>MAHHHHHHHHHHSGRAEDKSKRDSIEMSMKGCQTNNGFVHNEDILEQTPDPGSSTDNLKHSTRGILGSQEPDFKGVQPYAGMPKEVLFQFSGQARYRIPREILFWLTVASVLVLIAATIAIIALSPKCLDWWQEGPMYQIYPRSFKDSNKDGNGDLKGIQDKLDYITALNIKTVWITSFYKSSLKDFRYGVEDFREVDPIFGTMEDFENLVAAIHDKGLKLIIDFIPNHTSDKHIWFQLSRTRTGKYTDYYIWHDCTHENGKTIPPN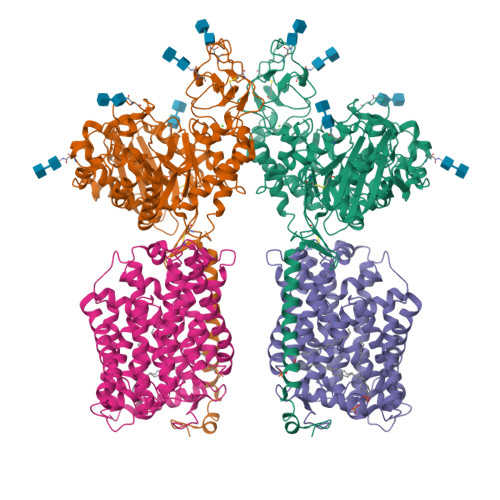NWLSVYGNSSWHFDEVRNQCYFHQFMKEQPDLNFRNPDVQEEIKEILRFWLTKGVDGFSLDAVKFLLEAKHLRDEIQVNKTQIPDTVTQYSELYHDFTTTQVGMHDIVRSFRQTMDQYSTEPGRYRFMGTEAYAESIDRTVMYYGLPFIQEADFPFNNYLSMLDTVSGNSVYEVITSWMENMPEGKWPNWMIGGPDSSRLTSRLGNQYVNVMNMLLFTLPGTPITYYGEEIGMGNIVAANLNESYDINTLRSKSPMQWDNSSNAGFSEASNTWLPTNSDYHTVNVDVQKTQPRSALKLYQDLSLLHANELLLNRGWFCHLRNDSHYVVYTRELDGIDRIFIVVLNFGESTLLNLHNMISGLPAKMRIRLSTNSADKGSKVDTSGIFLDKGEGLIFEHNTKNLLHRQTAFRDRCFVSNRACYSSVLNILYTSC[2x];>MADYKDDDDKSGPDEVDASGRGDTGLRKRREDEKSIQSQEPKTTSLQKELGLISGISIIVGTIIGSGIFVSPKSVLSNTEAVGPCLIIWAACGVLATLGALCFAELGTMITKSGGEYPYLMEAYGPIPAYLFSWASLIVIKPTSFAIICLSFSEYVCAPFYVGCKPPQIVVKCLAAAAILFISTVNSLSVRLGSYVQNIFTAAKLVIVAIIIISGLVLLAQGNTKNFDNSFEGAQLSVGAISLAFYNGLWAYDGWNQLNYITEELRNPYRNLPLAIIIGIPLVTACYILMNVSYFTVMTATELLQSQAVAVTFGDRVLYPASWIVPLFVAFSTIGAANGTCFTAGRLIYVAGREGHMLKVLSYISVRRLTPAPAIIFYGIIATIYIIPGDINSLVNYFSFAAWLFYGLTILGLIVMRFTRKELERPIKVPVVIPVLMTLISVFLVLAPIISKPTWEYLYCVLFILSGLLFYFLFVHYKFGWAQKISKPITMHLQMLMEVVPPEEDPE[2x]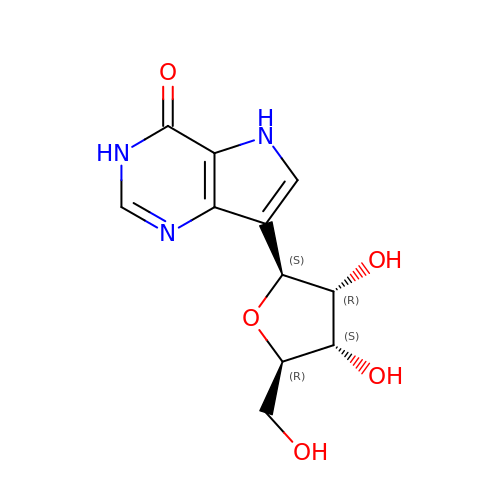9-DEAZAINOSINE | C11 H13 N3 O5 | WKDMPDYUJKSXBW-KBHCAIDQSA-N> EVARVRNLNRIIMGKYEIEPWYFSPYPIELTDEDFIYIDDFTLQYFGSKKQYERYRKKCTLRHPPGNEIYRDDYVSFFEIDGRKQRTWCRNLCLLSKLFLDHKTLYYDVDPFLFYCMTRRDELGHHLVGYFSKEKESADGYNVACILTLPQYQRMGYGKLLIEFSYELSKKENKVGSPQKPLSDLGLLSYRAYWSDTLITLLVEHQKEITIDEISSMTSMTTTDILHTAKTLNILRYYKGQHIIFLNEDILDRY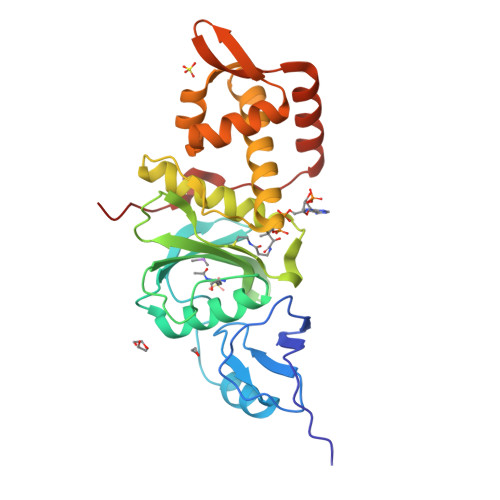NRLKAKKRRTIDPNRLIWKPPV>GPGSMTAEETVNVKEVEIIKLILDFLNSKKLHISMLALEKESGVINGLFSDDMLFLRQLILDGQWDEVLQFIQPLECMEKFDKKRFRYIILKQKFLEALCVNNAMSAEDEPQHLEFTMQEAVQCLHALEEYCPSK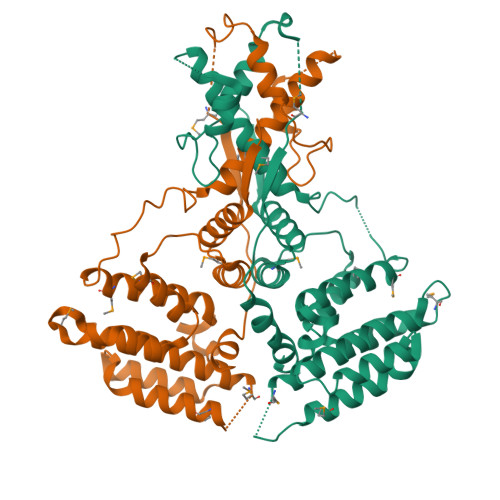DDYSKLCLLLTLPRLTNHAEFKDWNPSTARVHCFEEVCVMVAEFIPADRKLSEAGFKASNNRLFQLVMKGLLYECCVEFCQSKATGEEITESEVLLGIDLLCGNGCDDLDLSLLSWLQNLPSSVFSCAFEQKMLNIHVDKLLKPTKAAYADLLTPLISKLSPYPSSPMRRPQSADAYMTRSL[2x]> MIRRRLCFVSRPTKAASISVTLFSVQRQKGGLHTFIRDARSSSFTTPRQASHAEGEHTSSSLNSTDWATQMQRELFGETDPLGGQAHKDYYRDPARGYSPQYAPRNFAEGGAISYHHAQSPMEYAEATHRRSWLDHDVARMEAAFQEQRALLRGMESATERDELARRYAAEHHVADIVVENQSLLPSTQVHHSTSTSGSALRQQAVVDRFQIADQQSPLATSDGMGREELAHTYRMRSETVHNDWIEENLRIVHGLREKEKYDFTVLQRATRIPFQGYDMDRFLAQQKGTPYGAQSLPPNTASSTMEEAQRTLRDPTATVPSFEAISQKAFARNTVRDHPTTGEELTQEVVDTIRTSREASEWQREQERAQRFGLGRQGALVQDGGPDKRTLKKHVNDERIMDAMFFRSDAYRKTQTDEHWNPYMRQDTTHGVAHLLNNKFDIARREDRLSKGEQDLTERSVMHFGVPIQQTIDEFVFRHRNARGERPLDYFKPFPGFRDFRLNRMYRDVEGFSLMKQRPEFLEWELFTRYRAHHQQRRRIALLHGLEPVANETAQERDARREKLDEICERTPFDERELHTNDDEMQVSGETLRSWFGVYMLPSPTVVEAVVGASASVNLHLFPLADEMGTADTRENVLSSRYFNRLLLMEGFQNRISRAFMGNVSGKAPEPVVQYMQPPEVLRHFTAEERAMYEQYVKEQTSKQLGEWATAMRRRRWIPDRQQYGHVVAQGYGVSVVDLEHADTAAVLTVSAKAFERELAAAKGNTSHIIMVEGQAYKLRPDSERFVVPLSVRLESGEVLDMTDEAFGRYELELLPRNVNHALNYGIGDYAYNRGNYIETQDVIWEEQTASGEEGWSPATHADGLRAGLPVRARRHVGMNANGSRIVSSPQRAVIVAYDRQPFFNPEPRLVRVAFQSDGSVEEVPLANIMIWQRRYHGPERTVGDESRRFSPASLRRYIDVSDPFNEKKSKGEHFLDKYEAARTSEVAAGKYRTTKQITEIDQWTRFDVSRADNFRPLSISHRRDYIRLGYM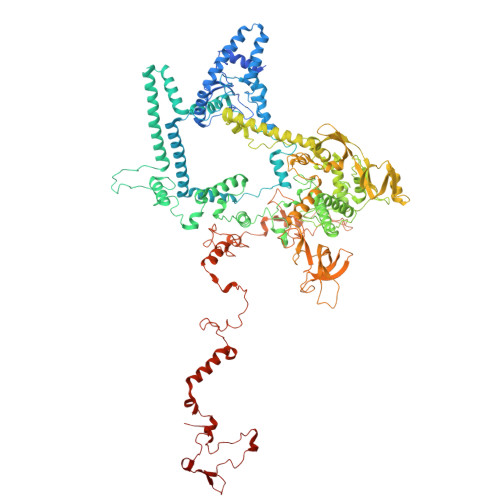HRYTPWEWIAVQEADQPLIAEQIRQDNIGTSYFFSLNRYWRYKARPHGYIRHFDNEVRDLFQFVDGVTPWKQAQKIRTYWEVRAHHPMPQFNRPEVAMHRNTVGLLPAHMWETDKKTGKVKAVKDSVRDYQTKTPLPKWVQL>[2x]MGSSHHHHHHSSGRENLYFQGMQKQILTSQKRNMYILSRCKVLVKNGQVCHLHEDGNVYTVPYANTVFIGLAEGTSITNEAMSMLAANGVIVFWTKGGGYDMFAADIICHLPQADYRPTKYMQNWVRLWLDEEKKLSAAKEILKMRVDSLSTHVHDFGVDVENKRVSSIVNKFDKGVTQATSFESLLGHEGTFVKSLYKEYALEYEIEFKRDHKSADNYNKFLTLGNYYA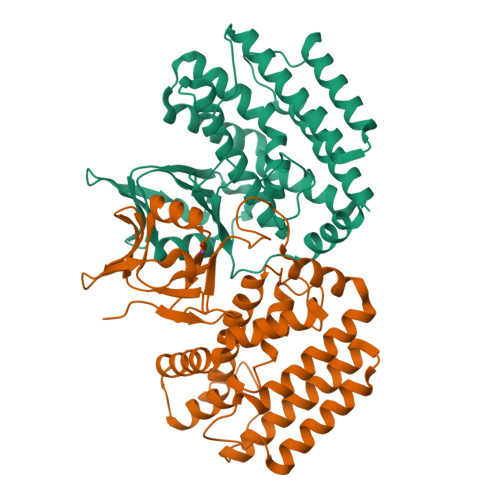YGIARSSLWALGIDNSFPLLHGSTRRGGLVFDVADIIKTSIILPLAFHAADQGMSNTEFKRSCVAYFDKNDILAYLINNIKRLCMENSDVHQD> ALRIDYPAALQILMEGGTHMVCTGRTHTDRICRFKWLCYSNEAEEFIFFHGNTSVMLPNLGSRRFQPALLDLSTVEDHATQYFNFVELPAAALRFMPKPVFVPDVALIANRFNPDNLMHVFHDDLLPLFYTLRQFPGLAHEARLFFMEGWGEGAHFDLYKLLSPKQPLLRAQLKTLGRLLCFSHAFVGLSKITTWYQYGFVQPQGPKANILVSGNEIRQFARFMTEKLNVSATGVPLGEEYILVFSRTQNRLILNEAELLLALAQEFQMKTVTVSLEDHTFADVVRLVSNASMLVSMHGAQLVTTLFLPRGATVVELFPYAVNPDHYTPYKTLAMLPGMDLQYVAWRNMMPENTVTHPERPWDQGGITHLDRAEQARILASREVPRHLCCRNPEWLFRIYQDTKVDIPSLIQTIRRVVKGRPGPRKQKWAAGLYPGKVREARCQASVHGASEARLTVSWQIPWNLKYLKVAEVKYEVWLQEAGEAAYVPYILALQNHTFTENIKPFTTYLVWVRCIFNKILLGPFADVLVCNT;> DYPAALQILMEGGTHMVCTGRTHTDRICRFKWLCYSNEAEEFIFFHGNTSVMLPNLGSRRFQPALLDLSTVEDHATQYFNFVELPAAALRFMPKPVFVPDVALIANRFNPDNLMHVFHDDLLPLFYTLRQFPGLAHEARLFFMEGWGEGAHFDLYKLLSPKQPLLRAQLKTLGRLLCFSHAFVGLSKITTWYQYGFVQPQGPKANILVSGNEIRQFARFMTEKLNASHTGVPLAEEYILVFSRTQNRLILNEAELLLALAQEFQMKTVTVSLEDHTFADVVRLVSNASMLVSMHGAQLVTTLFLPRGATVVELFPYAVNPDHYTPYKTLAMLPGMDLQYVAWRNMMPENTVTHPERPWDQGGITHLDRAQQAAILQSREVPRHLCCRNPEWLFRIYQDTKVDIPSLIQTIRRVVAAPGPAKQKAAAGLYPGKVREARCQASVHGASEARLTVSWQIPWNLKYLKVAEVKYEVWLQEQGEAAYVPYILALQNHTFTENIKPFTTYLVWVRCIFNKILLGPFADVLVCNT;> DYPAALQILMEGGTHMVCTGRTHTDRICRFKWLCYSNEAEEFIFFHGNTSVMLPNLGSRRFQPALLDLSTVEDHNTQYFNFVELPAAALRFMPKPVFVPDVALIANRFNPDNLMHVFHDDLLPLFYTLRQFPGLAHEARLFFMEGWGEGAHFDLYKLLSPKQPLLRAQLKTLGRLLCFSHAFVGLSKITTWYQYGFVQPQGPKANILVSGNEIRQFARFMTEKLNASHTGVPLAAEYILVFSRTQNRLILNEAELLLALAQEFQMKTVTVSLEDHTFADVVRLVSNASMLVSMHGAQLVTTLFLPRGATVVELFPYAVNPDHYTPYKTLAMLPGMDLQYVAWRNMMPENTVTHPERPWDQGGITHLDAAEQAAILQSREVPRHLCCRNPEWLFRIYQDTKVDIPSLIQTIRRVVKGAAPRKQAAAAGLYPGKVREARCQASVHGASEARLTVSWQIPWNLKYLKVAEVKYEVWLQEAGEAAYVPYILALQNHTFTENIKPFTTYLVWVRCIFNKILLGPFADVLVCNT;> ALRIDYPAALQILMEGGTHMVCTGRTHTDRICRFKWLCYSNEAEEFIFFHGNTSVMLPNLGSRRFQPALLDLSTVEDHNTQYFNFVELPAAALRFMPKPVFVPDVALIANRFNPDNLMHVFHDDLLPLFYTLRQFPGLAHEARLFFMEGWGEGAHFDLYKLLSPKQPLLRAQLKTLGRLLCFSHAFVGLSKITTWYQYGFVQPQGPKANILVSGNEIRQFARFMTEKLNASHTGVPLAAEYILVFARTQNRLILNEAELLAALAQEFQMKTVTVSLEDHTFADVVRLVSNASMLVSMHGAQLVTTLFLPRGATVVELFPYAVNPDHYTPYKTLAMLPGMDLQYVAWRNMMPENTVTHPERPWDQGGITHLDRAEQARILSSREVPRHLCCRNPEWLFRIYQDTKVDIPSLIQTIRRVVAGAPGPRKQKW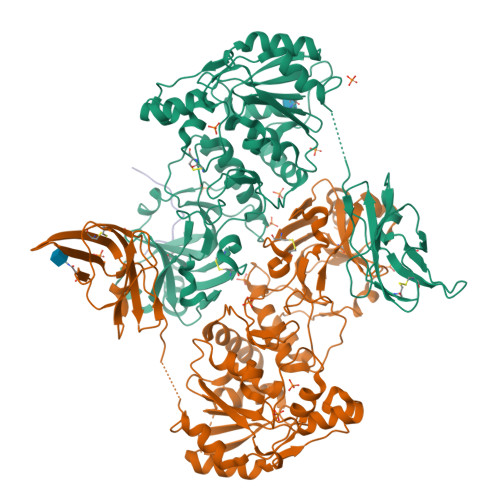TAGLYPGKVREARCQASVHGASEARLTVSWQIPWNLKYLKVAEVKYEVWLQEAGENTYVPYILALQNHTFTENIKPFTTYLVWVRCIFNKILLGPFADVLVCNT;> AAAAAAAAAA;> AGAGAAAAAA>[2x]SKVVYVSHDGTRRELDVADGVSLMQAAVSNGIYDIVGDCGGSAS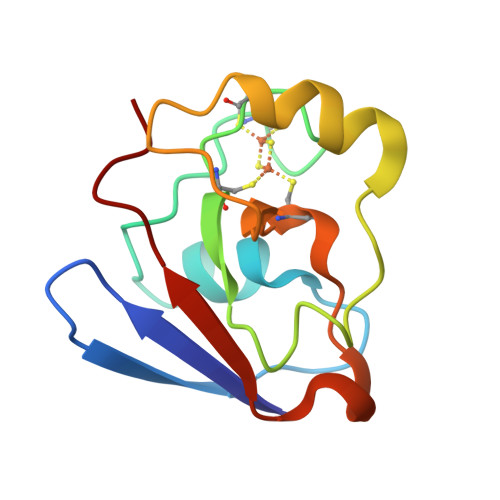CATCHVYVNEAFTDKVPAANEREIGMLESVTAELKPNSRLSCQIIMTPELDGIVVDVPDRQW L-gamma-glutamyl-S-benzyl-N-[(S)-carboxy(phenyl)methyl]-L-cysteinamide | C23 H27 N3 O6 S | 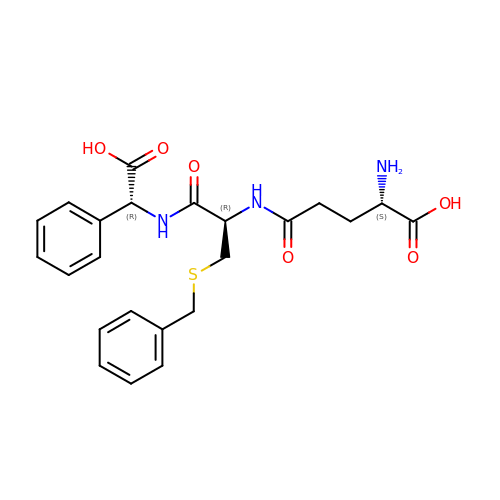ZPSKWMFLCHMEOY-CMKODMSKSA-N> MVYYPKKYELYKADEVPTEVVETDILIIGGGFSGCGAAYEAAYWAKLGGLKVTLVEKAAVERSGAVAQGLSAINTYIDLTGRSERQNTLEDYVRYVTLDMMGLAREDLVADYARHVDGTVHLFEKWGLPIWKTPDGKYVREGQWQIMIHGESYKPIIAEAAKMAVGEENIYERVFIFELLKDNNDPNAVAGAVGFSVREPKFYVFKAKAVILATGGATLLFRPRSTGEAAGRTWYAIFDTGSGYYMGLKAGAMLTQFEHRFIPFRFKDGYGPVGAWFLFFKCKAKNAYGEEYIKTRAAELEKYKPYGAAQPIPTPLRNHQVMLEIMDGNQPIYMHTEEALAELAGGDKKKLKHIYEEAFEDFLDMTVSQALLWACQNIDPQEQPSEAAPAEPYIMGSHSGEAGFWVCGPEDLMPEEYAKLFPLKYNRMTTVKGLFAIGDCAGANPHKFSSGSFTEGRIAAKAAVRFILEQKPNPEIDDAVVEELKKKAYAPMERFMQYKDLSTADDVNPEYILPWQGLVRLQKIMDEYAAGIATIYKTNEKMLQRALELLAFLKEDLEKLAARD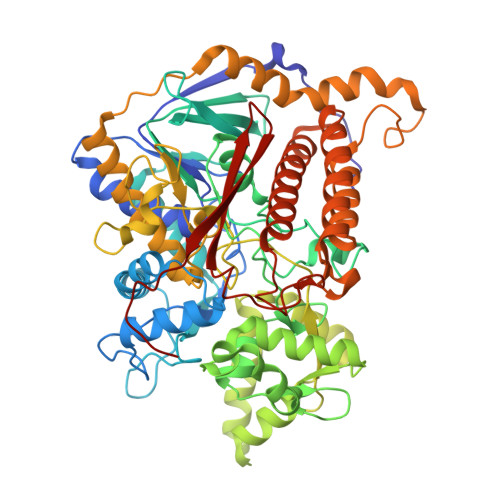LHELMRAWELVHRVWTAEAHVRHMLFRKETRWPGYYYRTDYPELNDEEWKCFVCSKYDAEKDEWTFEKVPYVQVIEWSF>GPHMGGSAEVNASPLKHFVTAKKKINGIFEQLGAYIQESATFLEDTYRNAELDPVTTEEQVLDVKGYLSKVRGISEVLARRHMKVAFFGRTSNGKSTVINAMLWDKVLPSGIGHTTNCFLRVEGTDGHEAFLLTEGSEEKRSAKTVNQLAHALHQDKQLHAGSLVSVMWPNSKCPLLKDDLVLMDSPGIDVTTELDSWIDKFCLDADVFVLVANSESTLMQTEKHFFHKVSERLSRPNIFILNNRWDASASEPEYMEEVRRQHMERCTSFLVDELGVVDRSQAGDRIFFVSAKEVLNARIQKAQGMPEGGGALAEGFQVRMFEFQNFERRFEECISQSAVKTKFEQHTVRAKQIAEAVRLIMDSLHMAAREQQVYCEEMREERQDRTRENLEQEIAAMNKKIEVLDSLQSKAKLLRNKAGWLDSELNMFTHQYLQPSR[4x]

Outer mitochondrial membrane (OMM) fusion is catalyzed by the dynamin-like GTPase called mitofusin (MFN). We generated a modified human MFN2 construct with deletions of residues 1–21 and 401–705 (MFN2IM). MFN2IM contains a G domain and a helical domain 1 (HD1). In this study, we address these issues by presenting crystal structures of truncated human MFN2 in different stages of the GTP turnover cycle. These structures explain how MFN2 uses a primate-only single amino acid variance and a tighter G interface, as compared with human MFN1, to allow for enduring GTPase (G) domain association even after GTP hydrolysis, a feature that is unique in the dynamin superfamily and ensures efficient membrane tethering.

We determined crystal structures of MFN2IM in the nucleotide-free and GDP-bound forms at 2.8 and 2.0 Å, respectively. Unlike MFN1, MFN2IM has a disordered switch I in the nucleotide-free state, and the Trp260 does not occupy the nucleotide-binding pocket. MFN2IM showed much higher affinity to GTPγS and GDP compared with MFN1IM, and could efficiently bind to GMPPNP. The stronger nucleotide association of MFN2IM may be partly explained by the aforementioned conformational variance to MFN1IM: the disordered switch I and outwardly oriented Trp260 leave an empty pocket that facilitates nucleotide docking. The cluster is apparently disfavored by the Thr129 exchange in MFN2, which endows the observed flexibility to switch I in the nucleotide-free state. Intriguingly, we observed calcium ions (Ca2+) associated with the HD1 of both nucleotide-free wild-type MFN2IM and MFN2IM(T111D), and one of them is involved in intermolecular contact. HD1 is connected to the G domain via the so-called hinge 2, namely Arg95 at the C-terminal end of α2H, and Lys357 between α5G and α3H. The four-helical-bundle HD1 is stabilized by a massive hydrophobic network. ɑ4H, which comprises large portion of the conventional HR2, is substantially involved in this network. The C-terminal tip of ɑ4H physically contacts the G domain. In our crystal structures, however, Met376 is surrounded by Phe56, Leu57, and Leu734 from the neighboring helices, and separated from Leu727.> IVGGTASVRGEWPWQVTLHTTSPTQRHLCGGSIIGNQWILTAAHCFYGVESPKILRVYSGILNQSEIAEDTSFFGVQEIIIHDQYKMAESGYDIALLKLETTVNYTDSQRPISLPSKGDRNVIYTDCWVTGWGYRKLRDKIQNTLQKAKIPLVTNEECQKRYRGHKITHKMICAGY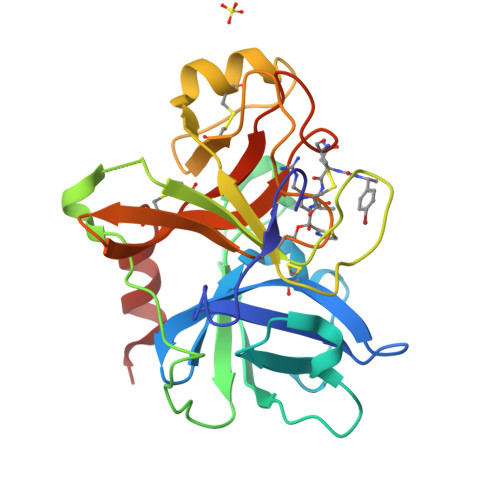REGGKDACKGDSGGPLSCKHNEVWHLVGITSWGEGCAQRERPGVYTNVVEYVDWILEKTQAV> QVVVLGYGTGQKLSTVSGSVAKVSSEKLAEKPVANIMDALQGQVAGMQVMTTSGDPTAVASVEIHGTGSLGASSAPLYIVDGMQTSLDVVATMNPNDFESMSVLKDASATSIYGARAANGVVFIQ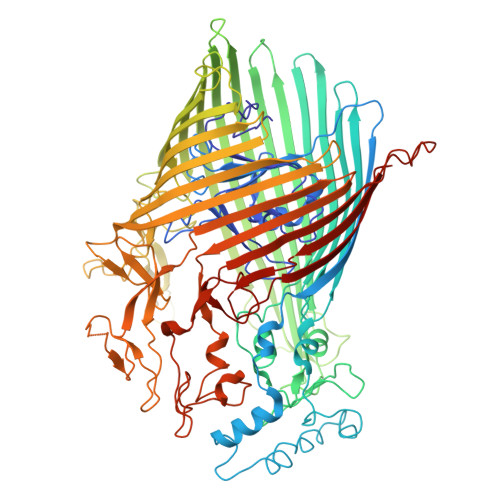TKKGKMSERGRITFNASYGISQILNTKPLDNMMTGDELLDFQVKAGFWGNNQTVQKVKDMILAGAEDLYGNYDSLKDEYGKTLFPVDFNHDADWLKALFKTAPTSQGDISFSGGSQGTSYYASIGYFDQEGMAREPANFKRYSGRLNFESRINEWLKVGANLSGAIANRRSADYFGKYYMGSGTFGVLTMPRYYNPFDVNGDLADVYYMYGATRPSMTEPYFAKMRPFSSESHQANVNGFAQITPIKGLTLKAQAGVDITNTRTSSKRMPNNPYDSTPLGERRERAYRDVSKSFTNTAEYKFSIDEKHDLTALMGHEYIEYEGDVIGASSKGFESDKLMLLSQGKTGNSLSLPEHRVAEYAYLSFFSRFNYGFDKWMYIDFSVRNDQSSRFGSNNRSAWFYSVGGMFDIYNKFIQESNWLSDLRLKMSYGTTGNSEIGNYNHQALVTVNNYTEDAMGLSISTAGNPDLSWEKQSQFNFGLAAGAFNNRLSAEVDFYVRTTNDMLIDVPMPYISGFFSQYQNVGSMKNTGVDLSLKGTIYQNKDWNVYASANFNYNRQEITKLFFGLNKYMLPNTGTIWEIGYPNSFYMAEYAGIDKKTGKQLWYVPGQVDADGNKVTTSQYSADLETRIDKSVTPPITGGFSLGASWKGLSLDADFAYIVGKWMINNDRYFTENGGGLMQLNKDKMLLNAWTEDNKETDVPKLGQSPQFDTHLLENASFLRLKNLKLTYVLPNSLFAGQNVIGGARVYLMARNLLTVTKYKGFDPEAGGNVGKNQYPNSKQYVAGIQLSF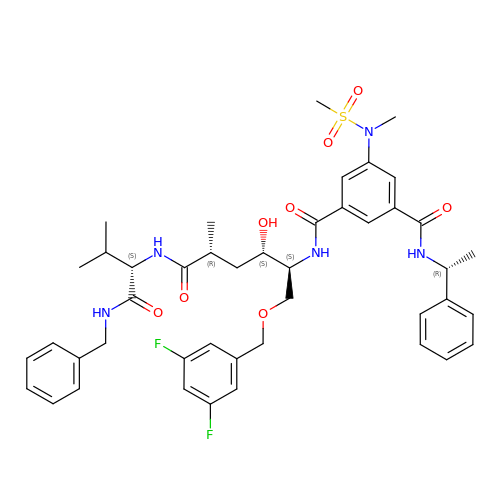N-[(2S,3S,5R)-1-[(3,5-difluorophenyl)methoxy]-3-hydroxy-5-methyl-6-[[(2S)-3-methyl-1-oxo-1-(phenylmethylamino)butan-2-yl]amino]-6-oxo-hexan-2-yl]-5-(methyl-methylsulfonyl-amino)-N'-[(1R)-1-phenylethyl]benzene-1,3-dicarboxamide | C44 H53 F2 N5 O8 S | SQCCLROLILAOBD-MLLWAOEYSA-N>MAMANNSSVANKVCLIVIDGWGVSEDPYGNAILNAQTPVMDKLCSGNWAQIEAHGLHVGLPEGLM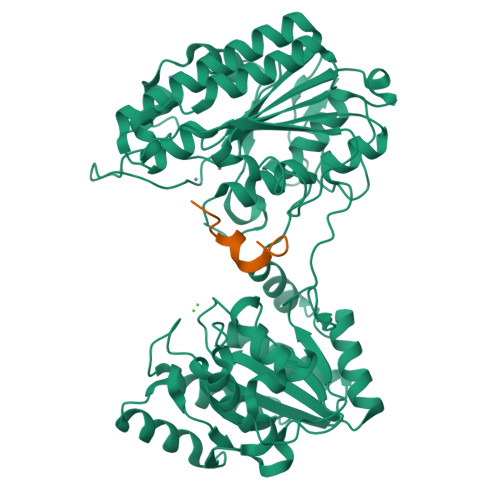GNSEVGHLNIGAGRVIYQDIVRINLAVKNNKFVTNESLVDACDRAKNGNGRLHLAGLVSDGGVHSHIDHMFALVKAIKELGVPELYLHFYGDGRDTSPNSGVGFLEQTLEFLEKTTGYGKLATVVGRYYAMDRDNRWERINVAYEAMIGGVGETSDEAGVVEVVRKRYAADETDEFLKPIILQGEKGRVQNDDTIIFFDYRADRMREISAAMGMDRYKDCNSKLAHPSNLQVYGMTQYKAEFPFKSLFPPASNKNVLAEWLAEQKVSQFHCAETEKYAHVTFFFNGGLEKQFEGEERCLVPSPKVATYDLQPEMSAAGVADKMIEQLEAGTHPFIMCNFAPPDMVGHTGVYEAAVKACEATDIAIGRIYEATQKHGYSLMVTADHGNAEKMKAPDGGKHTAHTCYRVPLTLSHPGFKFVDPADRHPALCDVAPTVLAIMGLPQPAEMTGVSIVQKIKLAAALEHHHHHHHHHH[2x];>XYDYPGDFCYLYGTCX[2x]>[3x]SGIRELNLTKEQHEWLNGWLELWGAWVYSGRLEKRMSSVIAKFMESVEPGRVMTRPMCNDDDGMLISQVVDSVMYIDKKAFGILLSYYAHGSSKHAIASYYHRVARPRKMLCRGGGRIQKP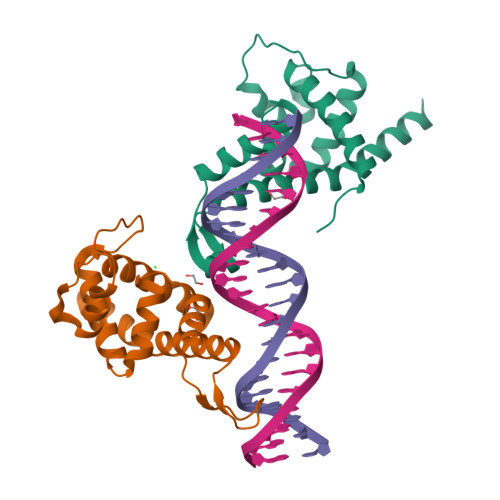SLATCRREVDEILNASLFMIYPVLDSAFKNRKRVEKIKHVA> MLEQPYLDLAKKVLDEGHFKPDRTHTGTYSIFGHQMRFDLSKGFPLLTTKKVPFGLIKSELLWFLHGDTNIRFLLQHRNHIWDEWAFEKWVKSDEYHGPDMTDFGHRSQKDPEFAAVYHEEMAKFDDRVLHDDAFAAKYGDLGLVYGSQWRAWHTSKGDTIDQLGDVIEQIKTHPYSRALIVSAWNPEDVPTMALPPCHTLYQFYVNDGKLSLQLYQRSADIFL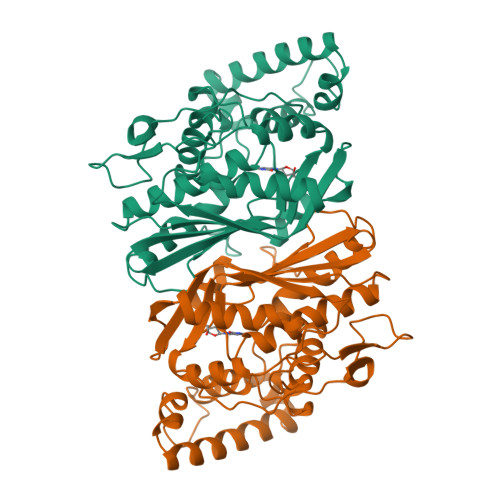GVPFNIASYALLTHLVAHECGLEVGEFIHTFGDAHLYVNHLDQIKEQLSRTPRPAPTLQLNPDKHDIFDFDMKDIKLLNYDPYPAIKAPVAV>PPGPPGPPGPPGP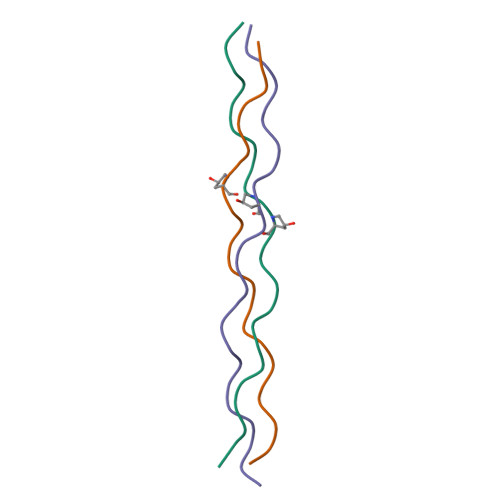PGPPGPPGPPGPPG[6x]> MEQVADFDTIYQAMIQISVVLCFALGIIA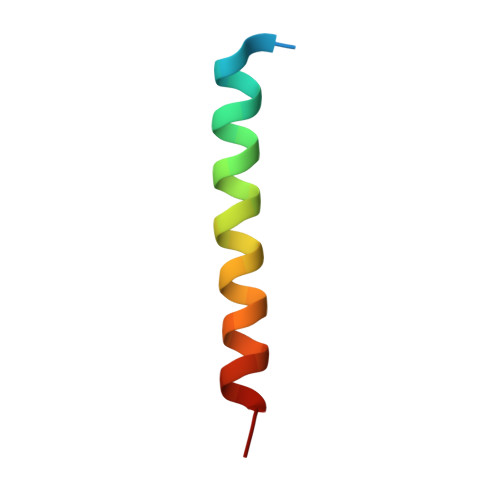GGQR> GPHMGSPEFDGTLVRIWMPDGAPA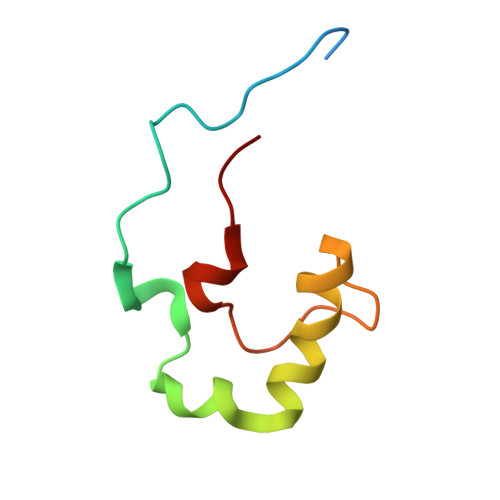YTADTEAEDPKVYEDEGVKRQWQSFLEKGRFEGGMPEVPPRREWCVWDF RIBOFLAVIN | C17 H20 N4 O6 | 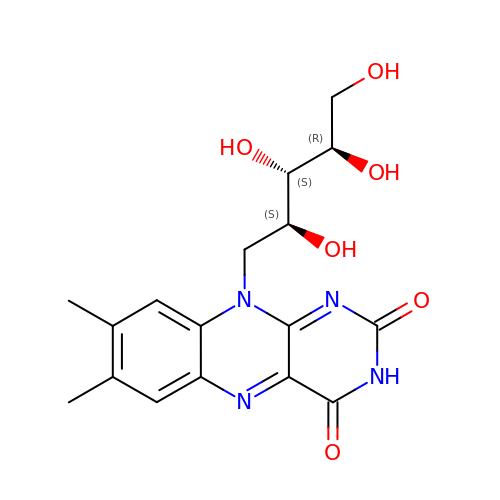AUNGANRZJHBGPY-SCRDCRAPSA-N> IDLGTGPTPTL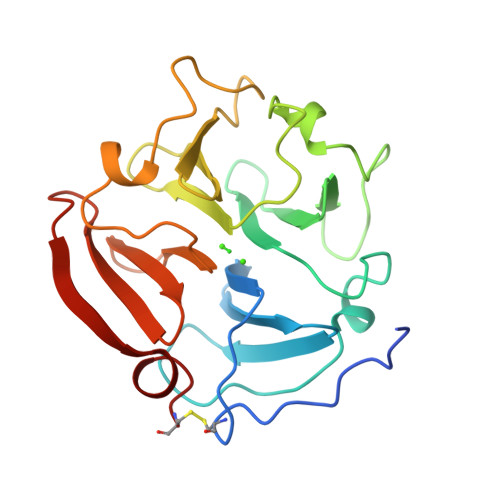GPVTPEICKQDIVFDGIAQIRGEIFFFKDRFIWRTVTPRDKPMGPLLVATFWPELPEKIDAVYEAPQEEKAVFFAGNEYWIYSASTLERGYPKPLTSLGLPPDVQRVDAAFNWSKNKKTYIFAGDKFWRYNEVKKKMDPGFPKLIADAWNAIPDNLDAVVDLQGGGHSYFFKGAYYLKLENQSLKSVKFGSIKSDWLGC> GDLADRFAELERRYDARLGVYVPATGTTAAIEYRADERFAFCSTFKAPLVAAVLHQNPLTHLDKLITYTSDDIRSISPVAQQHVQTGMTIGQLCDAAIRYSDGTAANLLLADLGGPGGGTAAFTGYLRSLGDTVSRLDAEEPELNRDPPGDERDTTTPHAIALVLQQLVLGNALPPDK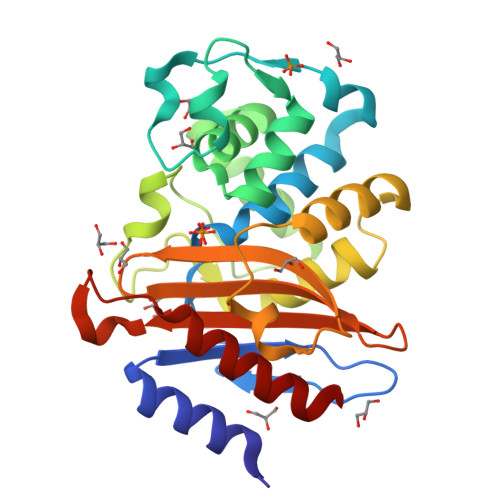RALLTDWMARNTTGAKRIRAGFGADWKVIDKTGTGDYGRANDIAVVWSPTGVPYVVAVMSDRAGGGYDAEPREALLAEAATCVAGVLA> GSPCELLPVGVGHPVQA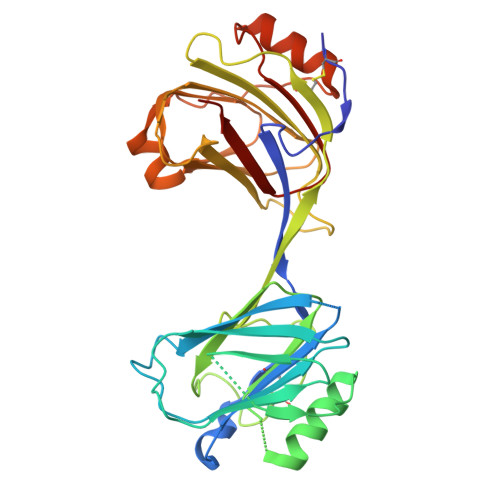MLKSFTALSGCASRGTTSHPQEVHIINLRKGSAQGAREKTAEVALHLRPIQSLHVHQKPLVFILNSPQPILWKVRTEKLAPGVKRIFHVVEGSEVHFEVGNFSKSCEVKVETLPHGNEHLLNWAHHRYTAVTSFSELRMAHDIYIKVGEDPVFSETCKIDNKFLSLNYLASYIEPQPSTGCVLSGPDHEQEVHIIELQAPNSSSAFQVDVIVDLRPLDGDIPLHRDVVLLLKCEKSVNWVIKAHKVMGKLEIMTSDTVSLSEDTERLMQVSKTVKQKLPAGSQALIQWAEENGFNPVTSYTNTPVANHFNLRLREHHHHHH> MGKREYPSSAHFLVTLSLLLLQAAFGLTLCIEKERDALLEFKRGLSDNFGQLSTWGDEEDKKECCKWKGIECNKTTGHVIVLDLHNAFTCSASACFAPRLTGKLSPSLLELEYLNFLDLSVNEFERSEIPRFICSFKRLEYLNLSSSFFSGLIPTQFKNLTSLRILDLGYNNLIVKDLTWLSHLSSLELLS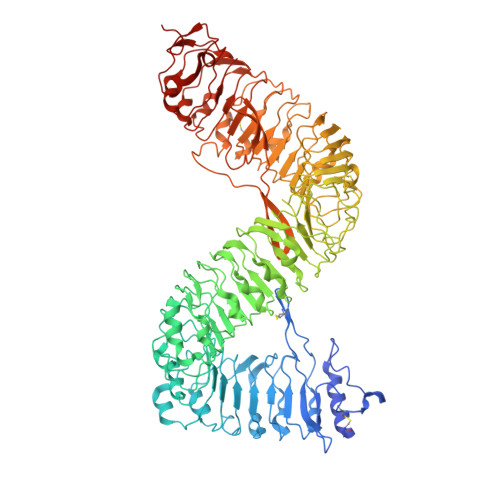LGGSDFQVKNWFQEITKLPLLKELDLSLCGLSKLVPSPAEIANSSLISLSVLHLCCNEFSSSAKYSWLFNFSTSLTSIDLSNNQLDGQIDDRFGNLMYLEHLNLANELNLKGGIPSSFGNLTRLRYLDMSNTRTYQWLPELFVRLSGSRKTLEVLGLNDNSMFGSLVDVTRFSALKRLYLQKNVLNGFFMERFGQVSSLEYLDLSDNQMRGPLPDLALFPSLRELHLGSNHFNGRIPQGIGKLSQLKILDVSSNRLEGLPESMGQLSNLESFDASYNVLKGTITESHLSNLSSLVDLDLSFNSLALKTSIDWLPPFQLQVINLPSCNLGPSFPKWLQSQNNYTVLDISLANISDALPSWFSGLPPDIKILNLSNNQISGRVSDLIENAYDYMVIDLSSNNFSGPLPLVPTNVQIFYLHKNQFFGSISSICKSTTGATSLDLSHNQFSGELPDCWMNATNLAVLNLAYNNFSGKLPQSLGSLTNLEALYMRQNSFSGMLPSLSQCQSLQILDLGGNKLTGRIPAWIGTDLLNLRILSLRFNKFYGSISPIICQLQFLQILDLSANGLAGKIPQCFNNFTLLHQENGLGEPMEFLVQGFYGKYPRHYSYLGNLLVQWKNQEAEYKNPLTYLKTIDLSSNKLVGGIPKEMAEMRGLKSLNLSRNDLNGSIIKGIGQMKMLESLDLSRNQLSGMIPKDLANLTFIGVLDLSNNHLSGRIPSSTQLQTFERSSYSGNAQLCGPPLQEC> KRPRTILTTQQRRAFKASFEVSSKPCRKVRETL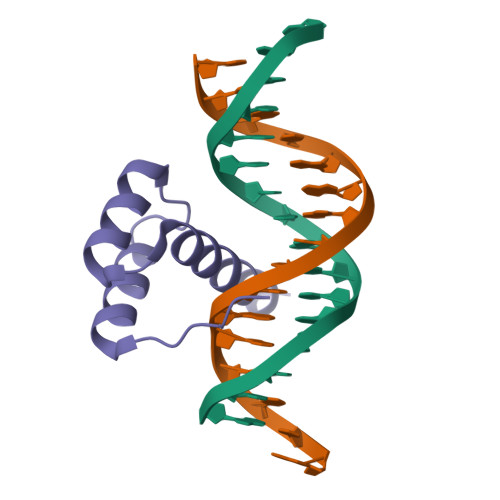AAETGLSVRVVQVWFQNQRAKMKKLAR(2S)-N,2-dicyclohexyl-2-[2-(2,4-dimethoxyphenyl)-1H-benzimidazol-1-yl]acetamide 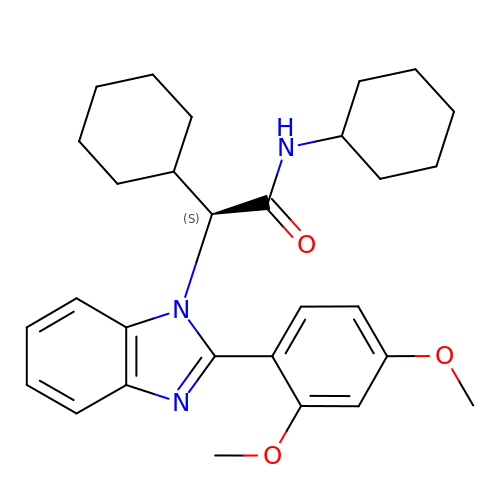| C29 H37 N3 O3 | VLEYYMSDWNFSEN-MHZLTWQESA-N> MGVSLSKGGNVSLTKEAPGLTAVIVGLGWDIRTTTGTDFDLDASALLLNSGGKVASDAHFIFFNNLKSPDGSVEHT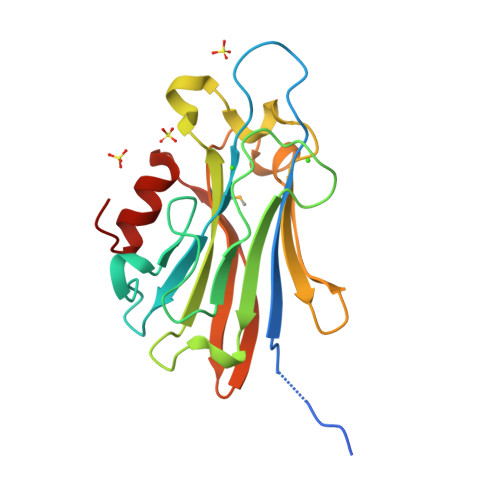GDNITGEGEGDDEQIKINLATVPADIEKIVFPVSIYDAENRQQSFGQVRNAFIRVVNQAGEAEIARYDLSEDASTETAMVFGELYRHGAEWKFRAIGQGYASGLRGIAQDFGVNV>MTADKKAKILATLGPATRSRDDIRALVEAGANLLRLNFSHGDYADHAQRFAWVREVEAELNYPIGVLMDLQGPKLRVGRFAAGAVQLQRGQTFTLDLSDAPGDERRVNLPHPEIIHALEPGMSLLLDDGKIRLEVVNCHSDAIETRVAVGGELSDRKGVNVPEAVLQLSPLTDKDRRDLAFGLELGVDWVALSFVQRPEDIDEARGLIGDKAFLMAKIEKPSAVSAIEAIAERADAIMVARGDLGVEVPAESVPGIQKRIVQVCRQLGKPVVVATQMLESMRFSPAPTRAEVTDVATAVGAGADAVMLSAETASGQYPREAVEMMAKIVRQVEAEPDYHVQLEVNRPQPDATVSDAISCAIRRVSRILPVAVLVNYTESGNSTLRAARERPKAPILSLTPNLRTARRLTVAWGVYSVVNEQLAHVDEICSTALDIALAQRMAR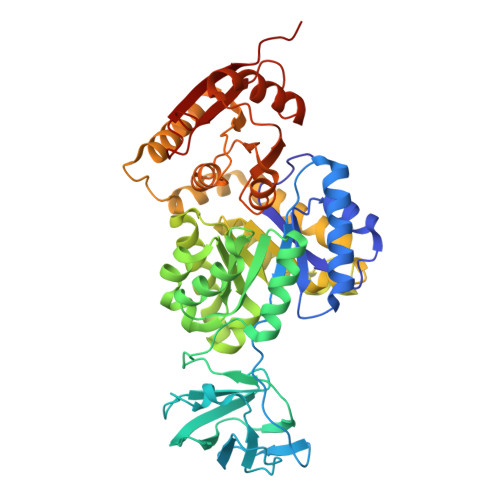RGDTVVVTAGVPFGRPGSTNMLRIETVAPPLGDL[2x]>PSVYDAAAQLTADVKKDLRDSWKVIGSDKKGNGVALMTTLFADNQETIGYFKRLGDVSQGMANDKLRGHSITLMYALQNFIDQLDNPDDLVCVVEKYAVNHITRKISAAEFGKINGPIKKVLASKNFGD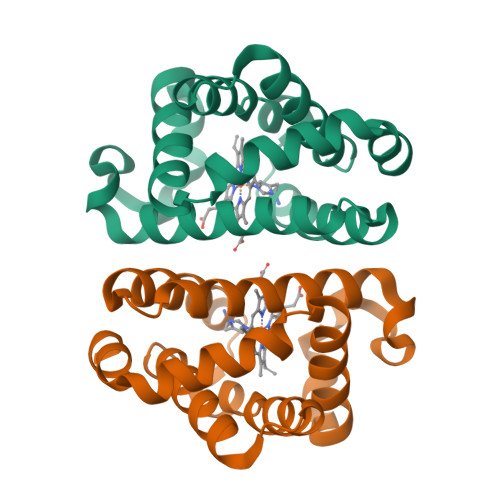KYANAWAKLVAVVQAAL[2x]(3aR,4S,4aR,7aR,8R,9aS)-4a,8-dimethyl-3-methylidene-2,5-dioxo-2,3,3a,4,4a,5,7a,8,9,9a-decahydroazuleno[6,5-b]furan-4-yl 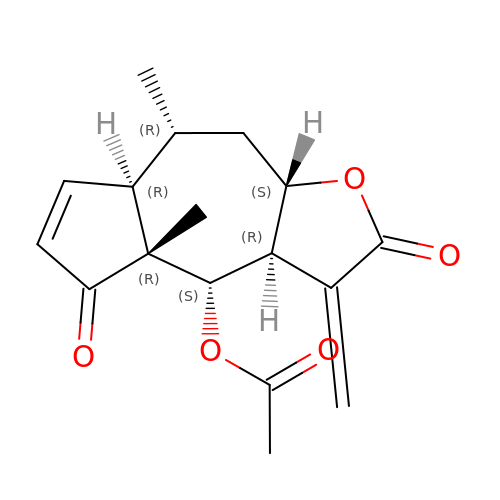acetate | C17 H20 O5 | DCNRYQODUSSOKC-MMLVVLEOSA-N> VVHVDTTLEKEDTLSYDNSDNMFCNKEYCNRLKDENNCISNLQVEDQGNCDTSWIFASKYHLETIRCMKGYEPTKISALYVANCYKGEHKDRCDEGSSPMEFLQIIEDYGFLPAE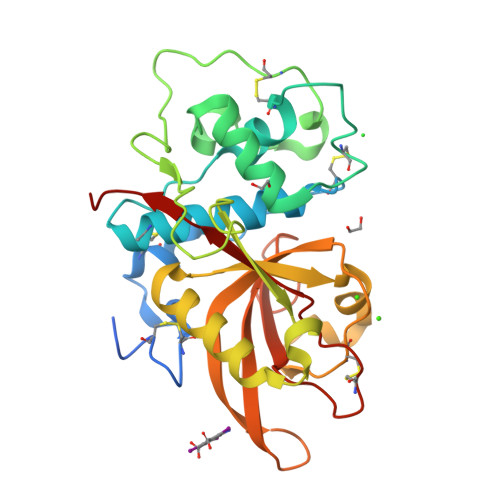SNYPYNYVKVGEQCPKVEDHWMNLWDNGKILHNKNEPNSLDGKGYTAYESERFHDNMDAFVKIIKTEVMNKGSVIAYIKAENVMGYEFSGKKVQNLCGDDTADHAVNIVGYGNYVNSEGEKKSYWIVRNSWGPYWGDEGYFKVDMYGPTHCHFNFIHSVVIFNVDLPMNN> MIEVKLRAIKRLSNVYTRRVMIIEDWNGSSITTGNIELVKGSENQLPQWLAIILEGKKVAKIEDKISIEDLGRILFQERQNMNTPASLVPLGKDFTSRVQLYLETLRKDNNVESLEKLRKSIGILNEIIKIRLRKLIQLAFLNIDDQNLINGMTEEELLIYKTIKQLIK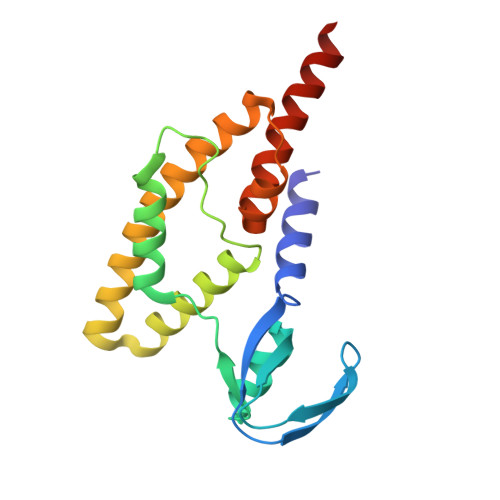ELYGDIIGNS>[2x]MEKLGDICFSLRYVPTAGKLTVVILEAKNLKKMDVGGLSDPYVKIHLMQNGKRLKKKKTTI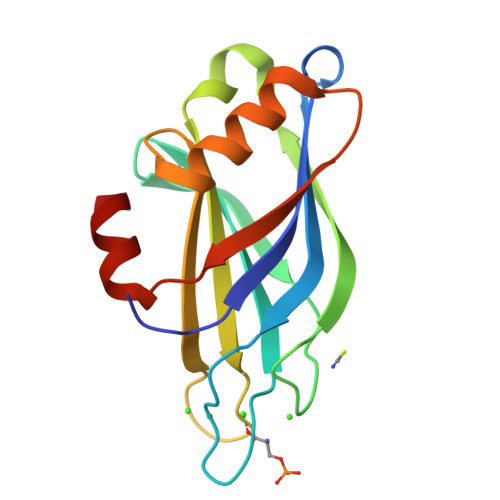KKNTLNPYYNESFSFEVPFEQIQKVQVVVTVLDYDKIGKNDAIGKVFVGYNSTGAELRHWSDMLANPRRPIAQWHTLQVEEEVDAMLAVKK>[4x]GPHMMIDLRSDTVTKPTEEMRKAMAQAEVGDDVYGEDPTINELERLAAETFGKEAALFVPSGTMGNQVSIMAHTQRGDEVILEADSHIFWYEVGAMAVLSGVMPH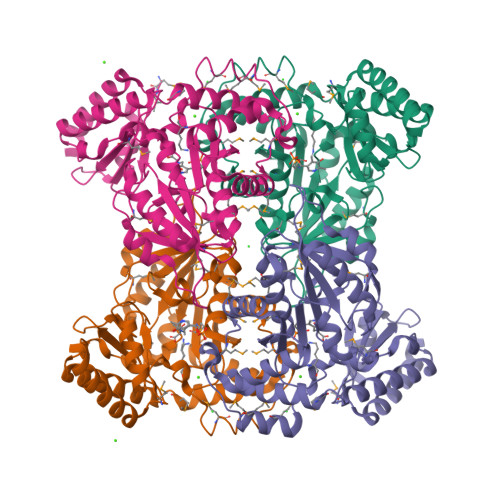PVPGKNGAMDPDDVRKAIRPRNIHFPRTSLIAIENTHNRSGGRVVPLENIKEICTIAKEHGINVHIDGARIFNASIASGVPVKEYAGYADSVMFCLSKGLCAPVGSVVVGDRDFIERARKARKMLGGGMRQAGVLAAAGIIALTKMVDRLKEDHENARFLALKLKEIGYSVNPEDVKTNMVILRTDNLKVNAHGFIEALRNSGVLANAVSDTEIRLVTHKDVSRNDIEEALNIFEKLFRKFS> GPLGSPEFPGRLEMEPDFFCVKWIPWKGEQTPIITQSTNGPCPLLAIMNILFLQWKVKLPPQKEVITSDELM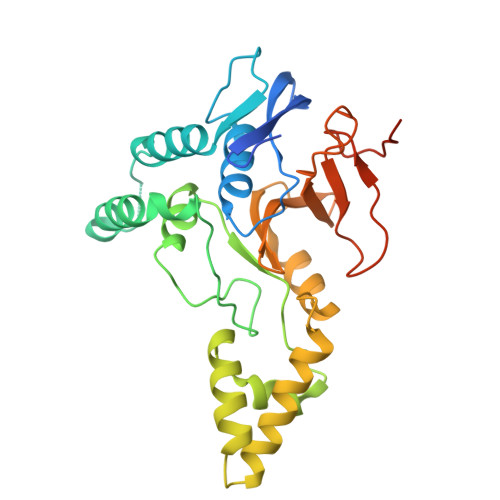AHLGNCLLSIKPQEKSEGLQLNFQQNVDDAMTVLPKLATGLDVNVRFTGVSDFEYTPECSVFDLLGIPLYHGWLVDPQSPEAVRAVGKLSYNQLVERIITCKHSSDTNLVTEGLIAEQFLETTAAQLTYHGLCELTAAAKEGELSVFFRNNHFSTMTKHKSHLYLLVTDQGFLQEEQVVWESLHNVDGDSCFCDSDFHLSHSLGKGPGAEGGSGSPE>PGSIPLIGERFPEMEVTTDHGVIKLPDHYVSQGKWFVLFSHPADFTPVCTTEFVSFARRYEDFQRLGVDLIGLSVDSVFSHIKWKEWIERHIGVRIPFPIIADPQGTVARRLGLLHAESATHTVRGVFIVDARGVIRTMLYYPMELGRLVDEILRIVKALKLGDSLKRAVPADWPNNEIIGEGLIVPPPTTEDQARARMESGQYRCLDWWFCWDTPASRDDVEEARR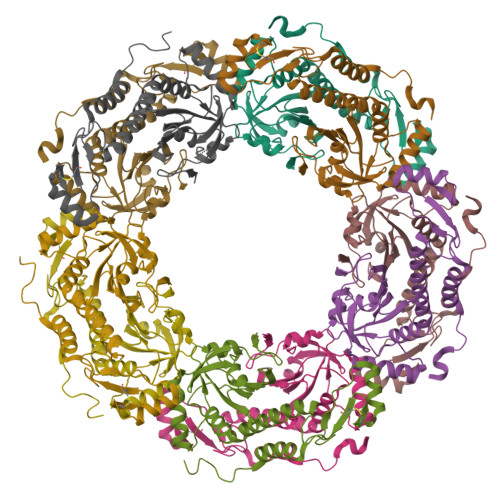YLRRAAEKPAKLLYEEARTHLH[10x]> LLQEEEEGLPLVGRVAAGEPLLAQQHIEGHYQVDPSLFKPNADFLLRVSGMAMKDIGIMDGDLLAVHKTQDVR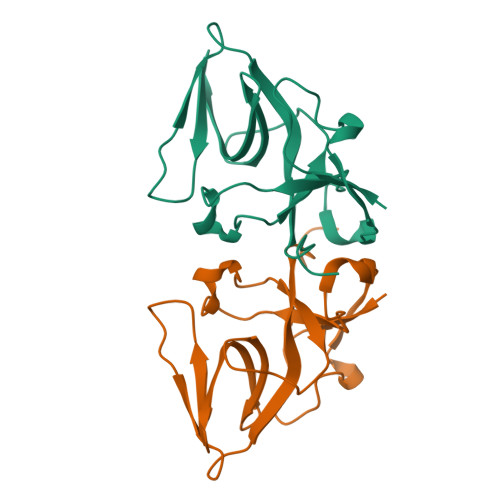NGQVVVARIDDEVTVKRLKKQGNKVELLPENSEFKPIVVDLRQQSFTIEGLAVGVIRNGDWLVP D-PHENYLALANYL-N~5~-[(2,2-DIHYDROXYHYDRAZINO)(IMINO)METHYL]-D-ORNITHINAMIDE | C15 H25 N7 O4 | 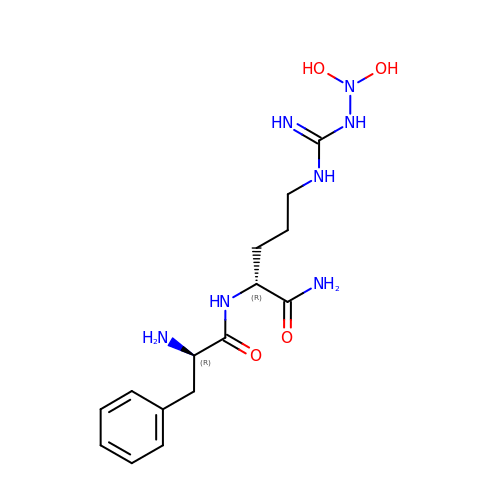XHGCEQHFMHULSW-VXGBXAGGSA-N>[4x]MGRKKIQITRIMDERNRQVTFTKRKFGLMKKAYELSVLCDCEIALIIFNSTNKLFQYASTDMDKVL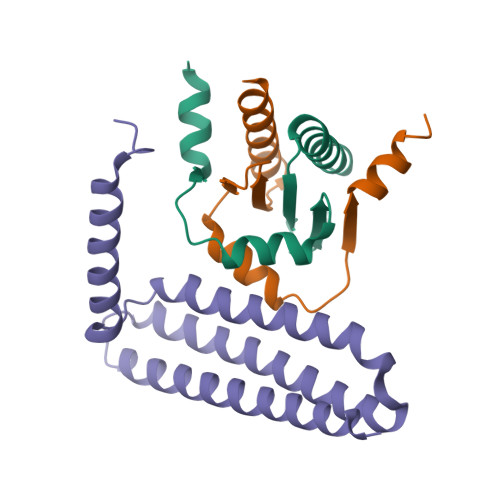LKYTEYNEPHESRTNSDIVEALNKKENKG;>LQPQEISPPPTANLDRSNDKVYENVTGLVKAVIEMSSKIQPAPPEEYVPMVKEVGLALRTLLATVDETIPALPASTHREIEMAQKLLNSDLGELISKMKLAQQYVMTSLQQEYKKQMLTAAHALAVDAKNLLDVIDQARLKMLGQTRPH[3x]>[2x]SMAKNRRDRNSWGGFSEKTYEWSSEEEEPVKKAGPVQVLIVKDDHSFELDETALNRILLSEAVRDKEVVAVSVAGAFAKGKSFLMDFMLRYMYNQESVDWVGDY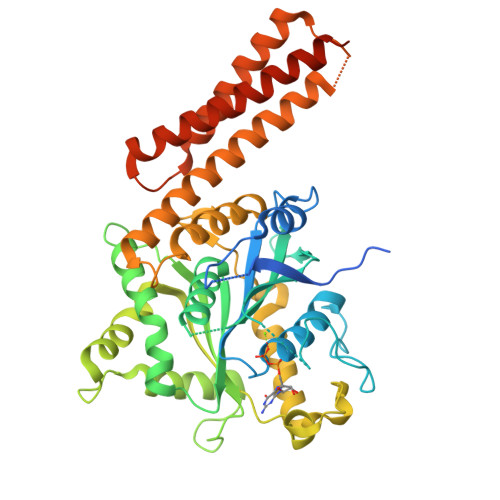NEPLTGFSWRGGSERETTGIQIWSEIFLINKPDGKKVAVLLMDTQGTSDSQSTLRDSATVFALSTMISSIQVYNLSQNVQEDDLQHLQLFTEYGRLAMEETFLKPFQSLIFLVRDWSFPYEFSYGADGGAKFLEKRLKVSGNQHEELQNVRKHIHSCFTNISCFLLPHPGLKVATNPNFDGKLKEIDDEFIKNLKILIPWLLSPESLDIKEINGNKITCRGLVEYFKAYIKIYQGEELPHPKSMLQATAEANNLAAVATAKDTYNKKMEEICGGDKPFLAPNDLQTKHLQLKEESVKLFRGVKKMGGEEFSRRYLQQLESEIDELYIQYIKHNDSKNIFHAARAAALEHHHHHH In this work, we investigate the mechanism of activity of anti-CRISPR protein AcrIIC2Nme. This 123-residue protein was previously shown to inhibit the activity of Neisseria meningitidis CRISPR-Cas9 in vivo and in vitro. We show that AcrIIC2Nme functions by inhibiting loading of the guide RNA molecule, thereby preventing formation of the active CRISPR-Cas9 surveillance complex. We found that it blocks Cas9 binding to sgRNA, thereby inhibiting biogenesis of the surveillance complex. This interference is mediated through an interaction with the arginine-rich bridge helix, which connects the REC lobe to the NUC lobe.

To better understand the precise mechanism by which AcrIIC2Nme inhibits Cas9 activity, we determined its crystal structure to a resolution of 2.5 Å using single-wavelength anomalous diffraction (SAD). Consistent with these previous observations, AcrIIC2Nme shares no sequence or structural similarity with previously characterized anti-CRISPR proteins. We also created a mutant lacking the final 12 amino acids (Δ112–123), which were not resolved in one of the apo crystal structures. The crystal structure of AcrIIC2Nme revealed a highly negatively charged surface that binds to the positively charged bridge helix. Mutation of this electronegative surface decreases the affinity of AcrIIC2Nme for Cas9, resulting in loss of anti-CRISPR activity. To determine if the interactions between AcrIIC2Nme and the bridge helix of Nme1Cas9 are required and sufficient for anti-CRISPR inhibitory activity, we mutated 19 residues distributed widely across the surface of AcrIIC2Nme. Mutation of three of the four amino acids that make direct contacts with the bridge helix (E17A, E24A, D108A) displayed a complete lack of anti-CRISPR activity in vivo while the other mutants showed changes in activity of less than 10-fold. Circular dichroism spectroscopy of the three mutants with abrogated in vivo activity revealed spectra similar to the wild type protein, showing that the lack of activity was not due to a folding defect. In addition, cooperative thermal denaturation curves and melting temperatures similar to the wild type protein indicated that these mutants maintained stable, folded structures. We conclude that the negatively charged surface of AcrIIC2Nme and the positively charged Nme1Cas9 bridge helix comprise a critical interaction interface that is required for anti-CRISPR activity.

>[3x]SMSKNNIFNKYPTIIHGEARGENDEFVVHTRYPRFLARKSFDDNFTGEMPAKPVNGELGQIGEPRRLAYDSRLGLWLSDFIMLDNNKPKNMEDWLGQLKAACDRIAADDLMLNEDAADLEGWDD> PISPIETVPVKLKPGMDGPKVKQWPLTEEKIKALVEICTEMEKEGKISKIGPENPYNTPVFAIKKKDSTKWRKLVDFRELNKRTQDFWEVQLGIPHPAGLKKKKSATVLDVGDAYFSVPLDEDFRKYTAFTIPSINNETPGIRYQYNVLPQGWKGSPAIFQSSMTKILEPFRKQNPDIVICQYMDDLYVGSDLEIGQHRTKIEELRQHLLRWGLTTPDKKHQKEPPFLWMGYELHPDKWTVQPIVLPEKDSWTVNDIQKLVGKLNWASQIYPGIKVRQLCKLLRGTKALTEVIPLTEEAELELAENREILKEPVHGV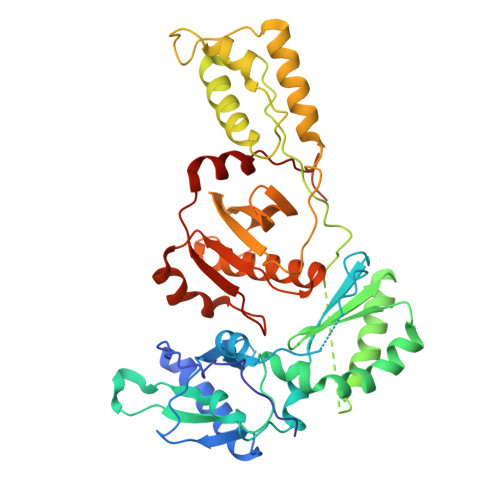YYDPSKDLIAEIQKQGQGQWTYQIYQEPFKNLKTGKYARMRGAHTNDVKQLTEAVQKITTESIVIWGKTPKFKLPIQKETWETWWTEYWQATWIPEWEFVNTPPLVKLWYQLEKEPIVGAETF>[2x]MAKSVIHQFFESGAKGDVDGAWACFADDAVWLASEGPEPGRTYTKTEIRDLLVQLDEMARTVRAQGMDGVFEEPVFLTDPDKAVVEWSLR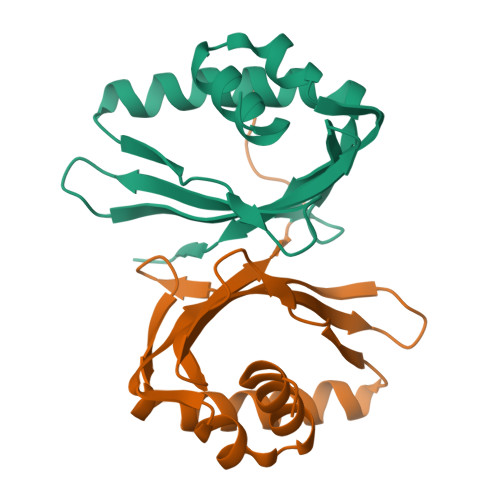KADGEVVDRGIDLFTLRDGKILVKDVFRKAKLAAALEHHHHHH4-(naphthalen-1-yl)-4-oxobutanoic acid | C14 H12 O3 | 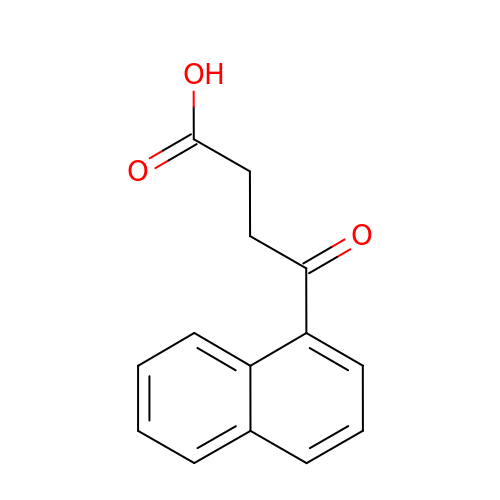YNEXYDHOGAIPHO-UHFFFAOYSA-N> GSGFTSKDTYLSHFNPRDYLEKYYKFGSRHSAESQILKHLLKNLFKIFCLDGVKGDLLIDIGSGPTIYQLLSACESFKEIVVTDYSDQNLQELEKWLKKEPAAFDWSPVVTYVCDLEGNRVKGPEKE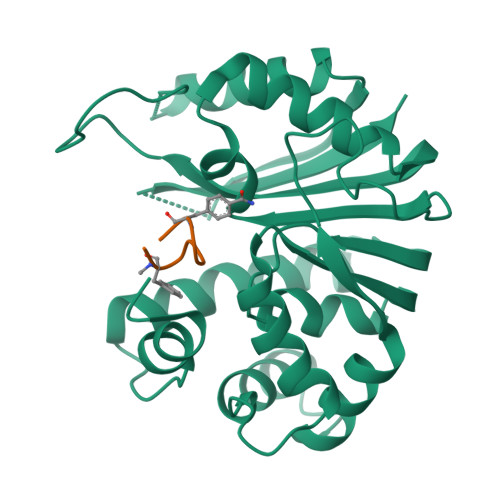EKLRQAVKQVLKCDVTQSQPLGAVPLPPADCVLSTLCLDAACPDLPTYCRALRNLGSLLKPGGFLVIMDALKSSYYMIGEQKFSSLPLGREAVEAAVKEAGYTIEWFEVISQSYSSTMANNEGLFSLVARKL;> GFPYRPXFC>[4x]NLFQFGEMILQKTGKEVVHSYAIYGCYCGWGGQGRAQDATDRCCFVHDCCYGTVNDCNPKTATYSYSFENGDIVCGDNDLCLRTVCECDRAAAIC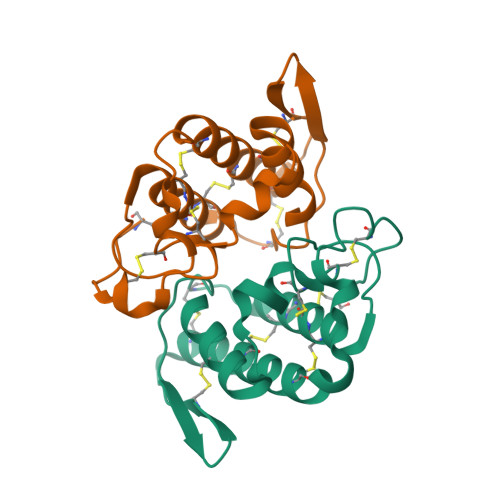LGQNVNTYDKNYEYYSISHCTEESEQC;>[4x]NLFQFARMINGKLGAFSVWNYISYGCYCGWGGQGTPKDATDRCCFVHDCCYGGVKGCNPKLAIYSYSFQRGNIVCGRNNGCLRTICECDRVAANCFHQNKNTYNKEYKFLSSSKCRQRSEQC>[2x]SNAMKHYLICFDVQHDKTRAKLSRLLEKYGPRVQGSVFEVSFKTPDRKRQLEYKIHQIIKQSNTEENNIRFYNLNKDTIKHSH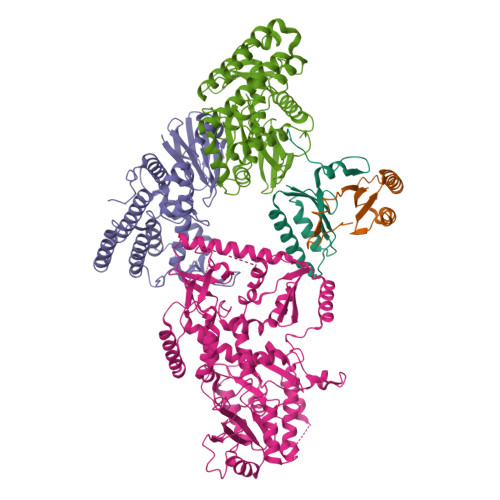DINGNPIAQLPAAIVL;>SNAMILPSFPDLTGLVVNLKFTARAEFSLNHEMAVDAFLRHSLNLGESYSHHLSIITPENGRLFYREGDTYRFVVIAMGNQQQTNSIWHTLINHLRKLPDSAPITDKQAPLRNNIKLESLNDLFDGIPVSSKESLDAYTLQRAMEQGLAWHKAANLTEQPLDIQWYWQSTVRILHADHKQHKGEQRYCRDAVQLTPLLLLKRIYETLNNVATYFGLKTNKNTTENHQAWLKEQAQYIEIQHPDLYWIDTPYFGKDAEKNTLGGMAGNFTLSLKPGIEPGLLAMLILTQMVGVGQRRTSGLGKYWLKHSLKHAHLILGLKPNRVTRSQTLLDCIIQPHIISQAIAEIEKKTNIDTLNERTLSQVQSAIGQLRKHQYQAPKLQGFTIPKKDGTERLLAVSPLYDRILQKAAAIVLTPGLDAIMSQASYGYRKGLSRQQVRYEIQNAYRQGYHWVYESDIEDFFDAVYRPQLINRLKSLLGNDPLWEQIESWLGQDIHIKDTIIERTPNLGLPQGSPLSPLLANFILDDFDSDLETHGFKIIRFADDFIILCKSQHEAQQAAHAVEQSLKEVKLSINVEKTHIIQLNQGFRFLGYLFREDHAIEIAGEKSDGRTTFAAEQTPTNLPPWLANLGTKSPQPLADDDLPKKSYGQIETQGTHLVLAGDAQIITTDNQNLIVKKDDKITHKISLEQLHAVTLIGLHTMTLPAKHRLLEHKIPVHIADRTGRYLGAVTSFQPAQNNYKNWFIQLQMCDREPFAHAIAQQIVISRIHNQRQTLLKRKAHRKQLQQTLSNLKKLQYKVTAATKRSSLNGLEGSATREYFQQFNLFLPEWAHFSKRTRRPPKDPFNVLLSLGYTILYSHTDAILQSAGFITWKGIYHQQSAAHAALASDIMESYRHLVERYAIYIINHGQIKQDDFRQEKDHLGQDTIRLSAEARRRYVGGLINRFQKFSKDKTLHQHLYQQAQQLKNAMHNQQSSQFQVWKELK[3x]> SKTAKIDWSHWTVTVPEENPDKPGKPYSLGYPEILNYAEDKIASKYMYDDPKDKSVVFYAFPSGVTTANTHYSRSELRETMETGSNKVNWTFAKGGKMRGTYAIDDISKEPDGKYSRVIIAQIHGVLTDEQRD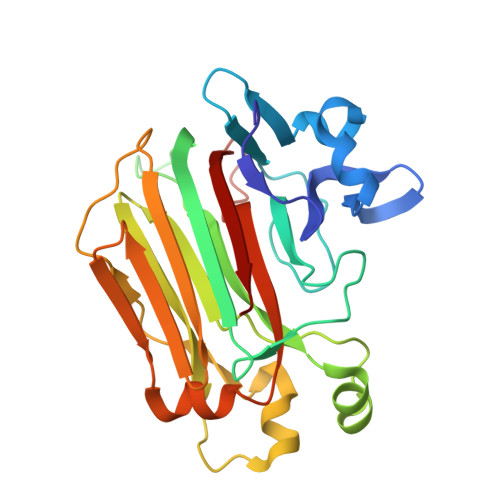LIGQKDNNAPPILKVYWDKGKIRVKTKVLKDLNAPYKEMLSEHAWGGDEGRNFKEKIDLNTRFTLEVKVSDGRMEVILNDTESLVYDDIHMKKWGIFENYFKAGNYFQSKTPGTFAKVKIYSLQVTHL>CKGADGAHGVNGCPGTAGAAGSVGGPGCDGGHGGNGGNGNPGCAGGV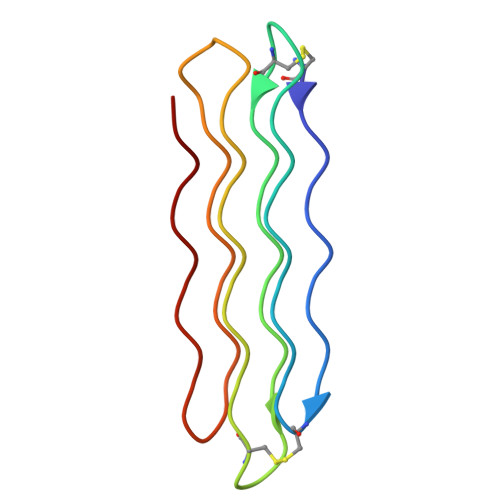GGAGGASGGTGVGGRGGKGGSGTPKGADGAPGAP[2x]>SMPVKKQEAHRALELLEDYHARLSEPQDRALRIAIERVIRIFKSRLFQALLDIQEFYELTLLDDSKSIQQKTAETLQIATKWEKDGQAVKIADF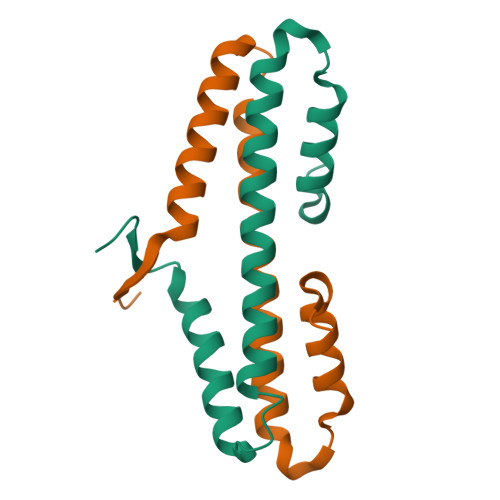IKSS[2x]> KSYVADSSGQTYYFDGNGQPLIGLQTIDGNLQYFNQQGVQIKGGFQDVNNKRIYFAPNTGNAVANTEIINGKLQGRDANGNQVKNAFSKDVAGNTFYFDANGVMLTGLQTISGKTYYLDEQGHLRKNYAGTFNNQFMYFDADTGAGKTAIEYQFDQGLVSQSNENTPHNAAKSYDKSSFENVDGYLTADTWYRPTDILKNGDTWTASTETDMRPLLMTWWPDKQTQANYLNFMSSKGLGITTTYTAATSQKTLNDAAFVIQTAIEQQISLKKSTEWLRDAIDSFVKTQANWNKQTEDEAFDGLQWLQGGFLAYQDDSHRTPNTDSGNNRKLGRQPINIDGSKDTTDGKGSEFLLANDIDNSNPIVQAEQLNWLHYLMNFGSITGNNDNANFDGIRVDAVDNVDADLLKIAGDYFKALYGTDKSDANANKHLSILEDWNGKDPQYVNQQGNAQLTMDYTVTSQFGNSLTHGANNRSNMWYFLDTGYYLNGDLNKKIVDKNRPNSGTLVNRIANSGDTKVIPNYSFVRAHDYDAQDPIRKAMIDHGIIKNMQDTFTFDQLAQGMEFYYKDQENPSGFKKYNDYNLPSAYAMLLTNKDTVPRVYYGDMYLEGGQYMEKGTIYNPVISALLKARIKYVSGGQTMATDSSGKDLKDGETDLLTSVRFGKGIMTSDQTTTQDNSQDYKNQGIGVIVGNNPDLKLNNDKTITLHMGKAHKNQLYRALVLSNDSGIDVYDSDDKAPTLRTNDNGDLIFHKTNTFVKQDGTIINYEMKGSLNALISGYLGVWVPVGASDSQDARTVATESSSSNDGSVFHSNAALDSNVIYEGFSNFQAMPTSPEQSTNVVIATKANLFKELGITSFELAPQYRSSGDTNYGGMSFLDSFLNNGYAFTDRYDLGFNKADGNPNPTKYGTDQDLRNAIEALHKNGMQAIADWVPDQIYALPGKEVVTATRVDERGNQLKDTDFVNLLYVANTKSSGVDYQAKYGGEFLDKLREEYPSLFKQNQVSTGQPIDASTKIKQWSAKYMNGTNILHRGAYYVLKDWATNQYFNIAKTNE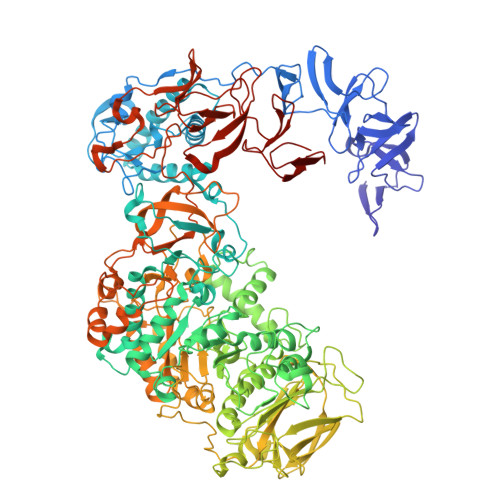VFLPLQLQNKDAQTGFISDASGVKYYSISGYQAKDTFIEDGNGNWYYFDKDGYMVRSQQGENPIRTVETSVNTRNGNYYFMPNGVELRKGFGTDNSGNVYYFDDQGKMVRDKYINDDANNFYHLNVDGTMS Although physiological activation of the MAPK pathway is RAS dependent, the interaction between RAS and the catalytic subunit of PI3Kα, p110α, serves as an amplifier but not a primary activator of this pathway, and is less important in normal cellular regulation than it is in cancer. Mutational studies have identified key residues, Thr208 and Lys227, within the RBD region of p110α, that facilitate interaction with RAS upon receptor tyrosine kinase-driven recruitment of PI3Kα to the plasma membrane. By mass-spectrometry-based chemoproteomics we detected 21 cysteines on p110α, including Cys242, which is exclusive to p110α, in the RBD and proximal to Thr208 and Lys227. We developed small molecules that covalently ligate Cys242, adjacent to the RAS binding interface of p110α, blocking its interaction with RAS proteins.

To understand how our covalent ligands for Cys242 blocked the interaction between RAS and p110α, we determined the X-ray co-crystal structure of VVD-442 covalently bound to the RBD of p110α at 2.83 Å resolution. The compound covalently bound to Cys242 in a hydrophobic groove between α-helices 3 and 4. The central sulfonamide formed a hydrogen bond with the terminal amide of Lys228, and the bromine formed a halogen bond (or σ-hole interaction) with a water positioned by Ser292. VVD-442 bound on the opposite side of β-strands 1 and 2 of the RBD, relative to the site of the primary interaction with RAS. Thus, we expect that the molecule does not block RAS-p110α binding through direct steric occlusion. Specifically, the positions of Arg230, Ser231 and Leu233 in the VVD-442 bound structure were incompatible with the switch I region of RAS observed in the p110α-RAS-glue complex. This model is consistent with experimental data showing that binding of VVD-442 to p110α disrupts the RAS-p110α interaction. VVD-699 and BBO-10203 are structurally distinct molecules, reflective of unique paths to discovery, leading to differing mechanisms by which they disrupt the RAS-PI3Kα interaction– VVD-699 binds adjacent to the RAS-p110α interface and stabilizes a conformation of the p110α RBD that is incompatible with RAS binding, whereas BBO-10203 induces a direct steric clash at the interface between RAS and p110α.

>[2x]NSPHSRAMYVYPPNVESSPELPKHIYNKLDKGQIIVVIWVIVSPNNDKQKYTLKINHDCVPEQVIAEAIRKKTRSMLLSSEQLKLCVLEYQGKYILKVCGCDEYFLEKYPLSQYKYIRSCIMLGRMPNLMLMAKESLYSQLPMD Zymogen granule membrane protein 16 (ZG16) is produced in organs that secrete large quantities of enzymes and other proteins into the digestive tract. ZG16 binds microbial pathogens, and lower ZG16 expression levels correlate with colorectal cancer, but the physiological function of the protein is poorly understood. One prominent attribute of ZG16 is its ability to bind glycans, but other aspects of the protein may also contribute to activity. An intriguing feature of ZG16 is a CXXC motif at the carboxy terminus.

Here, we describe crystal structures and biochemical studies showing that the CXXC motif is on a flexible tail, where it contributes little to structure or stability but is available to engage in redox reactions. ZG16 crystal structures also draw attention to a nonproline cis peptide bond that can isomerize within the protein and to the mobility of glycine‐rich loops in the glycan‐binding site. An understanding of the properties of the ZG16 CXXC motif and the discovery of internal conformational switches extend existing knowledge relating to the glycan‐binding activity of the protein.

> GARSSSYSGEYGSGGGKRFSHSGNQLDGPITALRVRVNTYYIVGLQVRYGKVWSDYVGGRNGDLEEIFLHPGESVIQVSGKYKWYLKKLVFVTDKGRYLSFGKDSGTSFNAVPLHPNTVLRFISGRSGSLIDAIGLHWDVYPTSCSRC> RQNWEEADSMKSSVESLQNRVTELESVDKSAGQVARNTGLLESQLSRHDQMLSVHDIRLADMDLRFQVLETASYNGVLIWKIRDYKRRKQE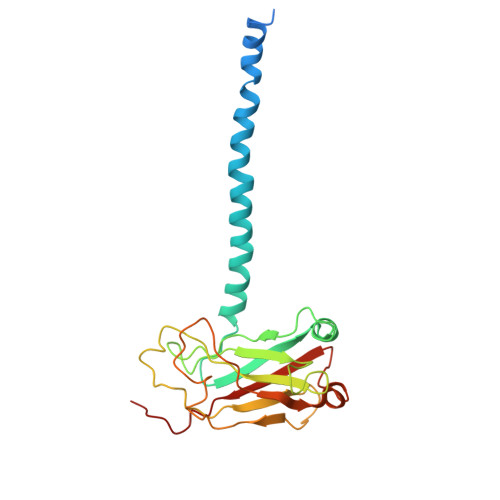AVMGKTLSLYSQPFYTGYFGYKMCARVYLNGDGMGKGTHLSLFFVIMRGEYDALLPWPFKQKVTLMLMDQGSSRRHLGDAFKPDPNSSSFKKPTGEMNIASGCPVFVAQTVLENGTYIKDDTIFIKVIVDTSDLPDP Ankyrins are a family of scaffold proteins which play essential roles in connecting numerous ion channels, cell adhesion molecules, and receptors to the spectrin-based cytoskeleton beneath membranes and thereby provide mechanical support for plasma membranes and control the activities of excitable tissues including neurons and muscles. There are three members in the human ankyrin family: ankyrin-R/B/G (AnkR/B/G) encoded by ANK1/2/3, respectively. They all consist of a highly similar N-terminal membrane binding domain composed of 24 ankyrin (ANK) repeats, a spectrin-binding domain comprised of two ZU5 domains, and a UPA domain followed by a death domain (DD) and a variable C-terminal regulatory domain. The wide-ranging physiological functions of ankyrins are the result of ankyrin's remarkable capacity for binding to and anchoring numerous membrane targets, via their N-terminal 24 ANK repeats, to specific membrane micro-domains in coordination with spectrin-based cytoskeletal structures. The 24 ANK repeats of ankyrins form a superhelical solenoid with an extremely conserved elongated inner groove, which contains multiple quasi-independent target binding sites.

Surprisingly, we found that the C-terminal part of the ABD (ABD-C, the 27-residue motif identified previously for ANK repeats binding) binds to ANK repeats with an affinity ∼15-fold weaker than the entire ABD, indicating that the ABD-C is not sufficient for binding to ANK repeats. We further showed that the ABD-C fragment binds to repeats 1–6 (R1–6) of ANK repeats, as ABD-C binds to R1–6 and the entire 24 ANK repeats with essentially the same affinities. Based on the structure of the ANK repeats/AS complex, we predicted that the Nav1.2_ABD-C may also bind to site 1 of AnkG_repeats with a pattern similar to the AS peptide. In the complex structure, the extended Nav1.2_ABD-C peptide interacts with the surface of the inner groove formed by the first five ANK repeats. In particular, the hydrophobic residues of Nav1.2_ABD-C and AS occupy very similar positions on the hydrophobic groove formed by residues from ANK repeats R4 and R5, and subtle conformational differences in the finger loops of R4 and R5 can accommodate amino acid sequence differences between the two targets. Unique to Nav1.2, the binding of ABD-C extends all the way to R1 via charge–charge and hydrogen-bond interactions. We noted that Glu1112, which is completely conserved in both Na+ and K+ channels and mutation of which in Nav1.5 to Lys is known to cause Brugada syndrome in humans, occupies the identical position as Glu1622 of AS does in the ANK repeats/AS complex. In contrast to the common expectation of directly interacting with positively charged residue(s), Glu1112 of Nav1.2 is buried deeply in the groove and forms hydrogen bonds with the sidechains of Thr94 and Asn98 in the R2 and R3 finger loop.

> GSTVTVPIAVGESDFENLNTEGSLVPRGSKSDSNASFLRAARAGNLDKVVEYLKGGIDINTCNQNGLNALHLAAKEGHVGLVQELLGRGSSVDSATKKGNTALHIASLAGQAEVVKVLVKEGANINAQSQNGFTPLYMAAQENHIDVVKYLLENGANQSTATEDGFTPLAVALQQGHNQAVAILLENDTKGKVRLPALHIAARKDDTKSAALLLQNDHNADVQSKMMVNRTTESGFTPLHIAAHYGNVNVATLLLNRGAAVDFTARNGITPLHVASKRGNTNMVKLLLDRGGQIDAKTRDGLTPLHCAARSGHDQVVELLKVVTEEVTT> MSQQENPKYLWWNHRIIPWEEATVHLTDYWWASVTAVFEVISGYWNNAEGEMYIFRLEDHARRLEQSMQLIRMPKEFTVDEICQATIDLVRANDYRGDVFIMPLAYAVGNKAFSVVGDRTTEMFIYSRPAVSRLEEDFSLHACYSSWTRINERVLPPRIKALANYRNSQLASSEAAMNGYDTALFLNPEGKVAEGTGSCVFFVRKGKLITPDITSGILESITRDTVIHLAREVLGLEVEERVVDRTETYLADEAFLCGTHAEITPIASIDRHEMKHGAPGPITRQLRDIYREVVYGRDFRYRNWLTPVGMGVRAEQ

Transaminases (TAs; aminotransferases; EC 2.6.1.) are pyridoxal-5’-phosphate (PLP)-dependent enzymes that catalyze the reversible stereoselective transfer of an amino group from an amino substrate to a keto acid or ketone, thereby producing a chiral amine or amino acid and a new keto compound. TaTT is distinguished by an expanded substrate specificity: it can catalyze the amino group transfer between BCAAs and α-ketoglutarate, producing α-keto acids and L-glutamate (benchmark reactions for BCATs), and between R-PEA and α-ketoglutarate producing ketone and L-glutamate (R-TA-like activity). The functional dimer of TaTT is close to the dimers of known BCATs; however, the P-pocket comprises only one site for the α-COOH group binding, and the O-pocket is enriched with hydrophobic residues, which disturb the alternation of hydrophobic and hydrophilic residues typical of BCATs. Generally, the active site is a combination of two pockets: the O-pocket on the phenolic side of the PLP and the P-pocket on the phosphate group side of the PLP.

The triple mutation G41V + Y101F + R43S (in mP3) destroyed the binding of the α-COOH group in TaTT and led to the loss of both BCAT-like and R-TA-like activities. However, triple mutation improved the affinity to R-PEA more than 60 times. When Y101 was substituted for phenylalanine, the side chain of the latter oriented almost 180° away from the P-pocket in both variants and accepted the conformation induced by both the R43S and G41V changes. The former created a void for phenyl moiety, occupied in WT TaTT by the R43 side chain, while the latter expelled the F101 side chain into this void. Compared to WT TaTT, the mP3 O-pocket loop lacks some stabilizing hydrogen bonds—between the backbone oxygen of S115* and the side chains of T197 and S173 and between the backbone oxygen of F114* and the side chain of Q170. These disturbances induced a shift of the loop, and thereby, the side chain of F114* shifted toward the cofactor and partially blocked the entrance into the active site. In WT TaTT, F114* is located opposite F39 and forms the stacking interactions with W32*, while in mP3, the side chain of W32* occupies the WT position of F114*. The triple mutation in the P-pocket induced a significant shift of the loop accompanied by a rearrangement of hydrogen bonding between the O-pocket loop and the structural elements forming the P-pocket. Consequently, the α-ketoglutarate binding sites are disturbed in mP3. Moreover, the side chain of F114* is placed in a potential position of the γ-COOH group and can prevent proper binding of α-ketoglutarate.> MEFTEFNLNELIREVYVLFEEKIRKMNIDFCFETDNEDLRVEADRTRIKQVLINLVQNAIEATGENGKIKITSEDMYTKVRVSVWNSGPPIPEELKEKIFSPFFTTKTQGTGLGLSICRKIIEDEHGGKIWTENREN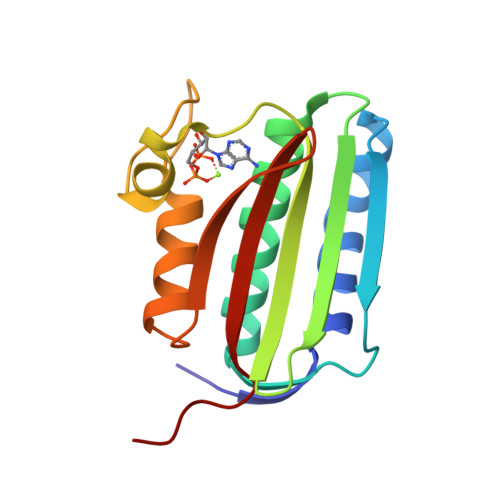GVVFIFEIPKTPEKR> GSELFRGVLQVSSNVLDCANDNWWCSLLDLDTSDWEPLTHTNRLMAIYLSSVASKLDFTGGPLAGCLYFFQVECNKFEEGYHIHVVIGGPGLNPRNLTVCVEGLFNNVLYHLVTGNVKLKFLPGMTTKGKYFRDGEQFIENYLMKKIPLNVVWCVTNIDGYIDTCISATFRRGACHA

The nuclease domain of NS1 (NS1_Nuc) is responsible for DNA Ori binding and nicking that is critical for B19V viral DNA replication. NS1 contains one nuclease domain (Nuc, aa 1–176), one helicase domain (aa 302–457) and one transactivation domain (TAD, aa 523–531). NS1 belongs to the HUH-endonuclease superfamily and it shares conserved ssDNA cleavage mechanism with other HUH-endonuclease members. NS1_Nuc is of α/β fold in nature.

Totally, two NS1_Nuc structures (Form I and Form II) were solved. The Form I structure belongs to P41212 space group; and, it was refined to final Rwork and Rfree of 18.0 % and 22.2 %, respectively. There is one NS1_Nuc molecule within the asymmetric unit. Except the extra Gly residue at the N-terminus and His175 and Ala176 at the C-terminus, all other residues are well ordered in the structure. The most distinctive conformation was observed for the β2-β3linker in the Form I structure. The main chain of Glu77 forms one hydrogen bond (H-bond) interaction with Asn74. The side chain of Glu77 forms two H-bond interactions: one with the main chain of Asn74 and the other with the side chain of His81 (one of the catalytic residues). Compared to the Form II structure, Glu77 is shifted about 7.3 Å in the Form I structure. However, mutagenesis and in vitro assay results suggested that Glu77 is not involved in direct DNA binding and cleavage by NS1_Nuc. Superposition showed that the overall folding of NS1_Nuc is very similar in the two structures; the root mean square deviation (RMSD) value is 0.8 Å, based on 169 pairs of Cα atoms.>HHHHHHFNLPPGNYKKPKLLYCSNGGHFLRILPDGTVDGTRDRSDQHIQLQLSAEENGEVYIKSTETGQYLAMDTDGLLYGSQTPNEECLFLERLEENHYNTYISK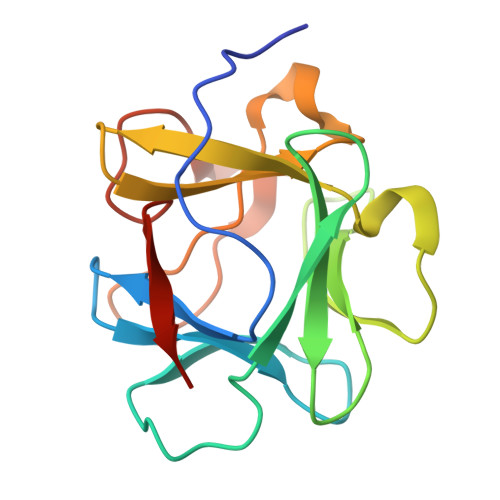KHAEKNWFVGLKKNGSCKRGPRTHYGQKAILFLPLPVSSD[2x]(2~{R})-2-[[5-(3-chloranyl-2-methyl-phenyl)-6-ethyl-thieno[2,3-d]pyrimidin-4-yl]amino]-3-phenyl-propanoic acid | C24 H22 Cl N3 O2 S | 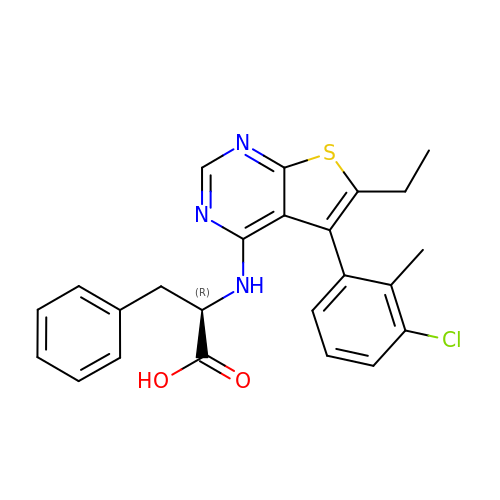MLKUMODNHNMDBV-GOSISDBHSA-N>QVGSSKNELETGSASNCPKAILIFARGSTETGNLGTLGAPLGDALESRYGASNVWVQGVGGPYDAALGDNALPRGSSAAAIREGVRLLNLANSKCPNSKVVAGGYSQGAALAAAAISDASTTVRNQIVGTVLFGYTKNQQNRGGIPGYPQDRLRVYCAVGDLVCEGTLIVLAPHLSYGDEARNEAP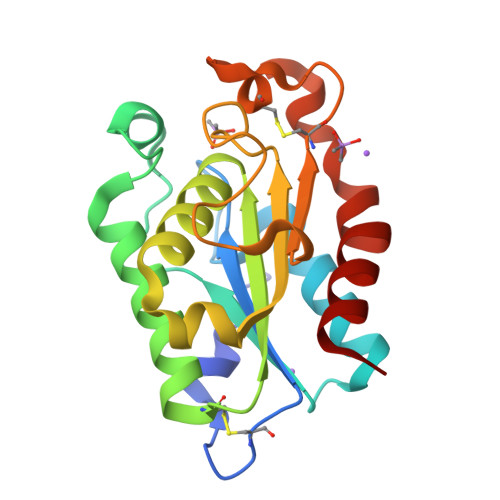AFLISKIGN[2x]(AMINOOXY)ACETIC 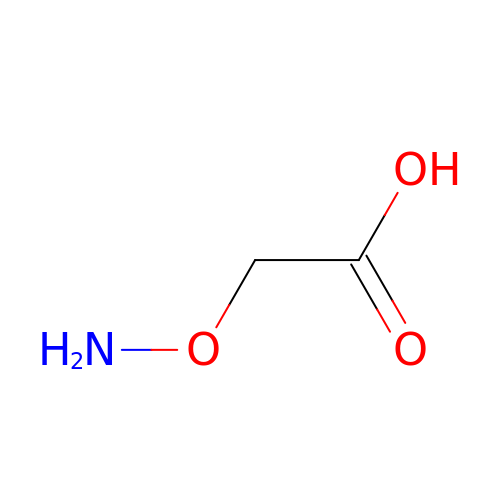ACID | C2 H5 N O3 | NQRKYASMKDDGHT-UHFFFAOYSA-N>[6x]SMTYETILVERDQRVGIITLNRPQALNALNSQVMNEVTSAATELDDDPDIGAIIITGSAKAFAAGADIKEMADLTFADAFTADFFATWGKLAAVRTPTIAAVAGYALGGGCELAMMCDVLIAADTAKFGQPEIKLGVLPGMGGSQRLTRAIGKAKAMDLILTGRTMDAAEA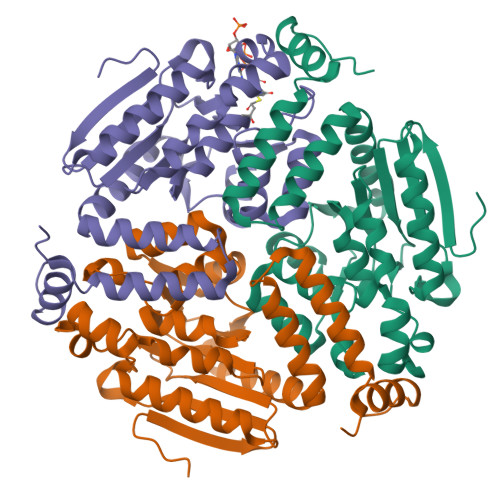ERSGLVSRVVPADDLLTEARATATTISQMSASAARMAKEAVNRAFESSLSEGLLYERRLFHSAFATEDQSEGMAAFIEKRAPQFTHR> MKIWSKEEVVNKLHEIKNKGYLSVPTDMFRTDDGVVGQILERQFGVQENNITLGDLGEFELKGMRNRKAKSNLTLFHKKPVAGQTVIQIFNRFGYVKPSSRNPEVMKKKLFTTIKGGRLNNLGLTLNAKHASEINLYYQDEYLSTWDLNLSKIEKLVLVFAETIGRANSPEEQFHFTKAYMLTEINDITSLINDGVLVMDLCIDQDLSKSKGPHDRGPH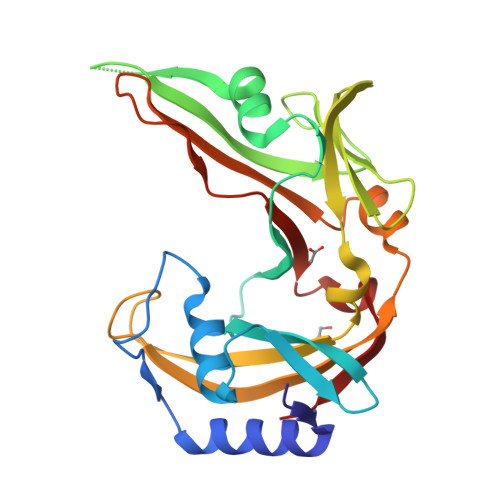LRIPISKLDKLYRNIERLL>MSDKIIHLTDDSFDTDVLKADGAILVDFWAEWCGPCKMIAPILDEIADEYQGKLTVAKLNIDQNPGTAPK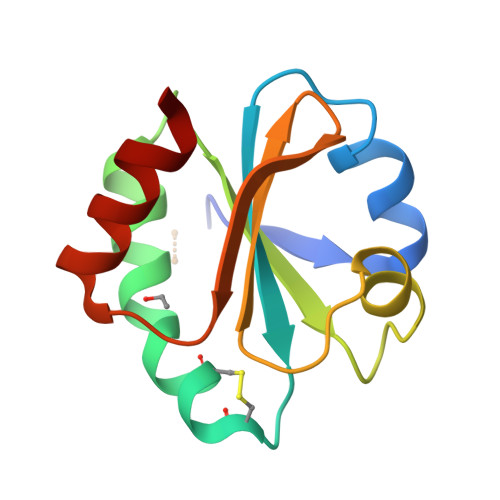YGIRGIPTLLLFKNGEVAATKVGALSKGQLKEFLDAALA[2x]>[2x]HLIPPLNFSMVDNGIFRSGFPDSANFSFLQTLGLRSIIYLCPEPYPESNLQFLKSNGIRLFQFGIEGNKEPFVNIPDHKIRMALKVLLDEKNHPVLIHCKRGKHRTGCLVG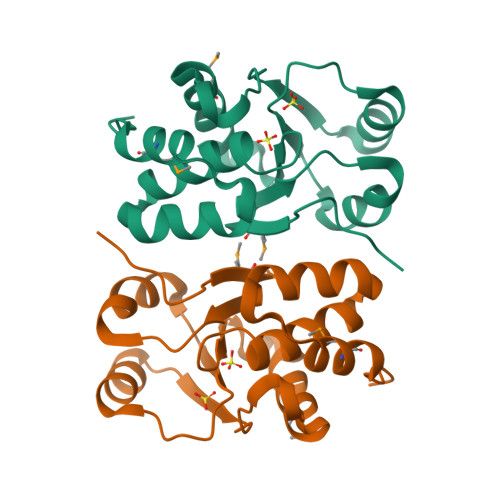CLRKLQKWCLTSIFDEYQRFAAAKARVSDQRFMEIFDVSS>MTEQTKKFPEGFLWGGAVAANQVEGAYNVGGKGLSTADVSPNGVMYPFDESMESLNLYHEGIDFYHRYKEDIALFAEMGFKAFRTSIAWTRIFPNGDETEPNEEGLEFYDRLFDELLKYNIEPVVTISHYEMPLGLIKKYGGWKNRKVIDCYEHYAKTVFTRYKEKVKYWMTFNEINMVLHAPFTGGGLVFEEGENKLNAMYQAAHHLFVASALAVKAGHDIIPDAKIGCMIAATTTYPMTPKPEDVLAAMENERRTLFFSDVQARGAYPGYMKRFFKENGITIEMAEGDEDILKENTVDYIGFSYYMSMVASTSPEDLAKTEGNLLGGVKNPYLESSEWGWQIDPKGIRITLNTLYDRYQKPLFIVENGLGAVDVVEEDGSIQD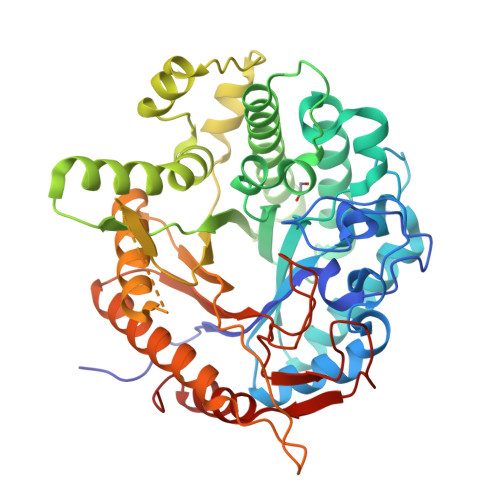DYRINYLRDHLKEVREAIADGVDLIGYTSWGPIDLVSASTAEMKKRYGYIYVDRDNEGKGTLSRTRKKSFYWYKKVIETNGESL[3x]(2S)-2-[3-(AMINOMETHYL)PHENYL]-3-[(S)-{(1R)-1-[(2,1,3-BENZOTHIADIAZOL-4-YLSULFONYL)AMINO]-2-METHYLPROPYL}(HYDROXY)PHOSPHORYL]PROPANOIC 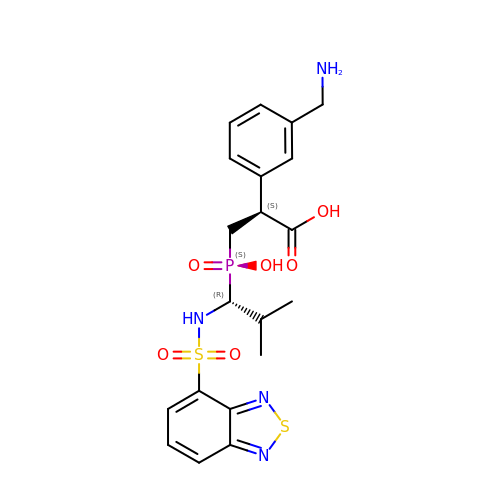ACID | C20 H25 N4 O6 P S2 | JQWWNMPDAALMKI-HNAYVOBHSA-N> MSQSSRLSALPIFQASLSASQSPRYIFSSQNGTRIVFIQDNIIRWYNVLTDSLYHSLNFSRHLVLDDTFHVISSTSGDLLCLFNDNEIFVMEVPWGYSNVEDVSIQDAFQIFHYSIDEEEVGPKSSIKKVLFHPKSYRDSCIVVLKEDDTITMFDILNSQEKPI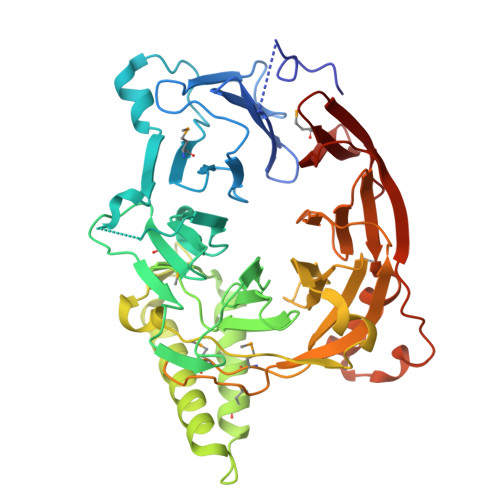VLNKPNNSFGLDARVNDITDLEFSKDGLTLYCLNTTEGGDIFAFYPFLPSVLLLNEKDLNLILNKSLVMYESLDSTTDVIVKRNVIKQLQFVSKLHENWNSRFGKVDIQKEYRLAKVQGPFTINPFPGELYDYTATNIATILIDNGQNEIVCVSFDDGSLILLFKDLEMSMSWDVDNYVYNNSLVLIERVKLQREIKSLITLPEQLGKLYVISDNIIQQVNFMSWASTLSKSINESDLNPLAGLKFESKLEDIATIERIPNLAYINWNDQSNLALMSNKTLTFQNISS>[4x]GSHMNGPIIMTREERMKIVHEIKERILDKYGDDVKAIGVYGSLGRQTDGPYSDIEMMCVMSTEEAEFSHEWTTGEWKVEVNFDSEEILLDYASQVESDWPLTHGQFFSILPIYDSGGYLEKVYQTAKSVEAQKFHDAICALIVEELFEYAGKWRNIRVQGPTTFLPSLTVQVAMAGAMLIGLHHRICYTTSASVLTEAVKQSDLPSGYDHLCQFVMSGQLSDSEKLLESLENFWNGI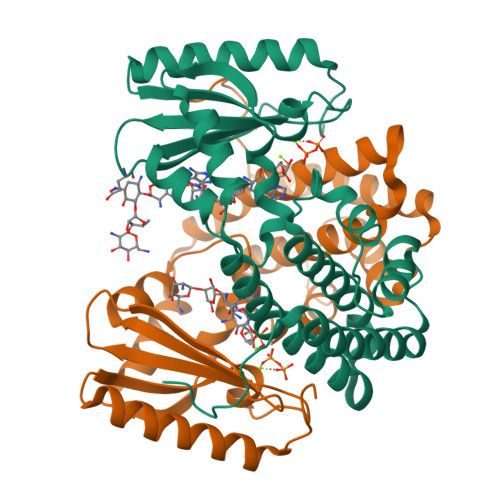QEWTERHGYIVDVSKRIPF1-[(2R)-3-[3,6-bis(fluoranyl)carbazol-9-yl]-2-oxidanyl-propyl]imidazolidin-2-one 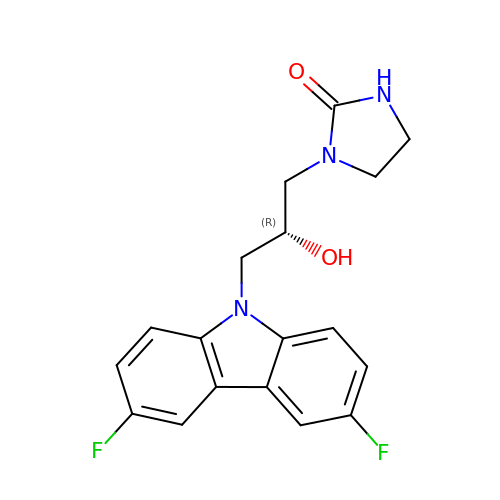| C18 H17 F2 N3 O2 | MUVYYQQLOKRDQS-ZDUSSCGKSA-N>NLKMEIILTLSQGLKKYYGKILRLLQLTLEEDTEGLLEWCKRNLGLDCDDTFFQKRIEEFFITGEGHFNEVLQFRTPGTLSTTESTPAGLPTAEPFKSYFAKGFLSIDSGYYSAKCYSGTSNSGLQLINITRHSTRIVDTPGPKITNLKTINCINLKASIFKEHREVEINVLLPQVAVNLSNCHVVIKSHVCDYSLDIDGAVRLPHIYHEGVFIPGTYKIVIDKKNKLNDRCTLFTDCVIKGREVRKGQSVLRQYKTEIRIGKASTGS[2x]

Crimean-Congo hemorrhagic fever virus (CCHFV) is the causative agent of the most widespread tick-borne viral infection in humans. CCHFV encodes a secreted glycoprotein (GP38) of unknown function that is the target of a protective antibody. Nairoviruses are the only bunyaviruses that are known to encode secreted glycoproteins, such as the 38-kDa glycoprotein (GP38) that is produced by CCHFV. GP38 (GPC residues 248 to 519) does not share substantial sequence homology with other viral or cellular proteins. It is N-glycosylated in the endoplasmic reticulum (ER) and cleaved by subtilisin kexin isozyme-1/site-1 protease (SKI-1/S1P) in the Golgi complex to liberate it from Gn.

We expressed a construct containing GPC residues 1 to 515 of CCHFV strain IbAr 10200 in FreeStyle 293 cells. Crystals of GP38 grew in 0.1 M sodium acetate (pH 5.5), 2% to 4% polyethylene glycol 400 (PEG 400), and 11% to 21% PEG 3350 and belonged to the P21 space group. Because GP38 lacks sequence homology to known structures, we collected multiple long-wavelength data sets on the beamline I23 at Diamond Light Source to obtain experimental phases via sulfur single-wavelength anomalous dispersion (SAD). The structure of GP38 was initially determined to 2.8 Å using these data sets, and was subsequently extended to 2.5-Å resolution with an additional data set collected at Advanced Photon Source. There are two molecules of CCHFV GP38 in the asymmetric unit, denoted chain A and chain B. Chain A has electron density for GPC residues 252 to 322 and 341 to 509, whereas chain B has electron density for GPC residues 250 to 327, 342 to 379, 387 to 486, and 499 to 514. The overall structure of GP38 is defined by a 3-helix bundle at the N terminus followed by a β-sandwich comprising 7- and 4-strand β-sheets. In addition to the β-sandwich, the β-strand-rich core of GP38 also contains a pair of small antiparallel β-strands. The region between residues 328 and 340 is disordered, suggesting that this loop is flexible. The CCHFV GP38 fold is stabilized by four disulfide bonds between Cys287 and Cys295, Cys363 and Cys439, Cys400 and Cys485, and Cys430 and Cys479. The CCHFV GP38 sequence contains N-linked glycosylation sequons at Asn376 and Asn426, and both of these sites showed well-resolved electron density for glycans extending away from the protein surface. No higher order oligomerization was detected from the crystallographic packing, consistent with the SEC data that GP38 is a monomer.> TAPSGSEYRHPGASDRPQPTAMNSIVMETGNTKNSALMAKKAPTMPKPQWHPPWKLYRVISGHLGWVRCIAVEPGNQWFVTGSADRTIKIWDLASGKLKLSLTGHISTVRGVIVSTRSPYLFSCGEDKQVKCWDLEYNKVIRHYHGHLSAVYGLDLHPTIDVLVTCSRDSTARIWDVRTKASVHTLSGHTNAVAT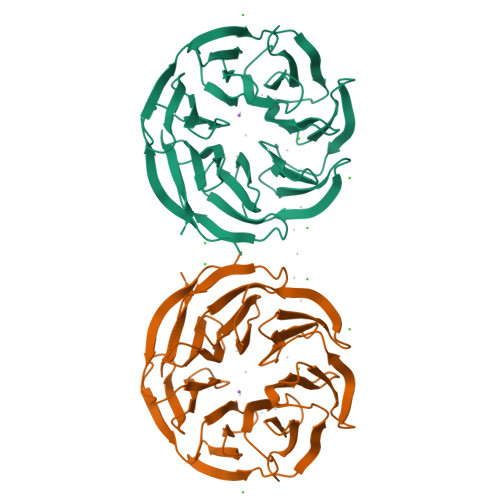VRCQAAEPQIITGSHDTTIRLWDLVAGKTRVTLTNHKKSVRAVVLHPRHYTFASGSPDNIKQWKFPDGSFIQNLSGHNAIINTLTVNSDGVLVSGADNGTMHLWDWRTGYNFQRVHAAVQPGSLDSESGIFACAFDQSESRLLTAEADKTIKVYREDDTATEETHPVSWKPEIIKRKRF The ganglioside-induced differentiation-associated protein 1 (GDAP1) is an integral MOM protein, proposed to have an auxiliary role in mitochondrial fission and fusion, possibly via redox-dependent interactions with cytoskeletal components. GDAP1 has two GST-like domains, followed by a transmembrane helix, which anchors the protein into the MOM. Structural data have shown a covalently bound dimer interface in GDAP1, and while dimerisation is a common feature in catalytic GSTs, the GDAP1 dimer is formed differently, with a unique interface having a central disulphide bridge between Cys88 from each subunit. We carried out structural and biophysical analyses on several CMT-linked GDAP1 protein variants and describe new crystal structures of the autosomal recessive R120Q and the autosomal dominant A247V and R282H GDAP1 variants.

R282H is located on helix α8, and the side chain of Arg282 points inwards in the wild-type GDAP1 structure; it is stacked against Trp238 and makes hydrogen bonds to the backbone carbonyl groups of residues 236 and 237 in the α6-α7 loop. All these interactions are lost upon the mutation, and the His residue in the mutant is observed in a double conformation, making no side-chain hydrogen bond contacts. Arg282, studied here in the form of the CMT mutation R282H, is one of the most conserved residues in the GDAP1/GDAP1L1 subfamily. Its strong hydrogen bonding to the carbonyl groups in the ⍺6-⍺7 loop indicates a central role in GDAP1 structure. Arg282 is, in addition, optimally stacked against the aromatic side chain of Trp238, which is both a conserved residue and a CMT mutation target itself. This Arg-Trp-(⍺6-⍺7) unit is likely important for the stable folding of GDAP1. In the case of Arg282, mutation to His is indeed one of the most destabilising variants in the prediction, linked to a loss of several key interactions by the Arg282 side chain. Arg282 in GDAP1 interacts directly with the backbone of the ⍺6-⍺7 loop, and a similar interaction is observed in GST. This is another example of an Arg–loop backbone interaction in GDAP1 that is both conserved and relevant for human disease mutations. Ab initio modelling, here carried out on the R282H mutant, which was measured at the highest concentration, supported the presence of a dimeric GDAP1, corresponding to the conformation of the dimer we previously showed to fit the solution SAXS data for wild-type GDAP1.

>EVKLILYHWTHSFSSQKVRLVIAEKALKCEEHDVSLPLSEHNEPWFMRLNSTGEVPVLIHGENIICEATQIIDYLEQTFLDERTPRLMPDKESMYYPRVQHYRELLDSLPMDAYTHGCILHPELTVDSMIPAYATTRIRSQIGNTESELKKLAEENPDLQEAYIAKQKRLKSKLLDHDNVKYLKKILDELEKVLDQVETELQRRNEETPEEGQQPWLCGESFTLADVSLAVTLHRLKFLGFARRNWGNGKRPNLETYYEHVLKRKTFNKVLGHVNNILIS[2x]> MEELQKSIGHKPEPTDEEWELIKTVTEAHVATNAQGSHWK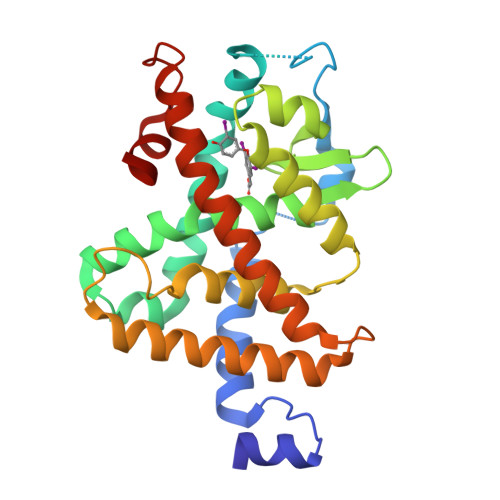QKRKFLPDDIGQAPIVNAPEGGKVDLEAFSHFTKIITPAITRVVDFAKKLPMFCELPCEDQIILLKGCCMEIMSLHAAVRYDPESETLTLNGEMAVTRGQLKNGGLGVVSDAIFDLGMSLSSFNLDDTEVALLQAVLLMSSDRPGLACVERIEKYQDSFLLAFEHYINYRKHHVTHFWPKLLMKVTDLRMIGACHASRFLHMKVECPTELFPPLFLEVFED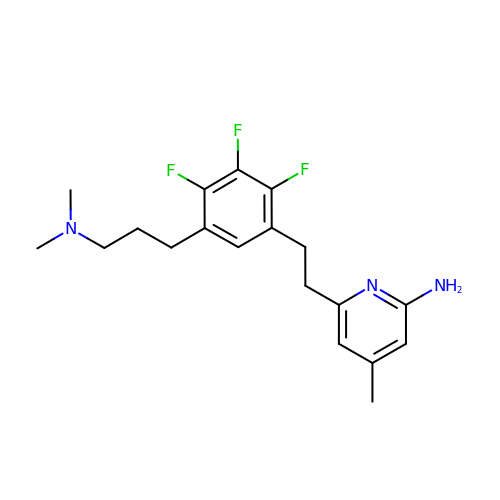6-(2-{5-[3-(dimethylamino)propyl]-2,3,4-trifluorophenyl}ethyl)-4-methylpyridin-2-amine | C19 H24 F3 N3 | QBZKHLSOLPLXGI-UHFFFAOYSA-N> IN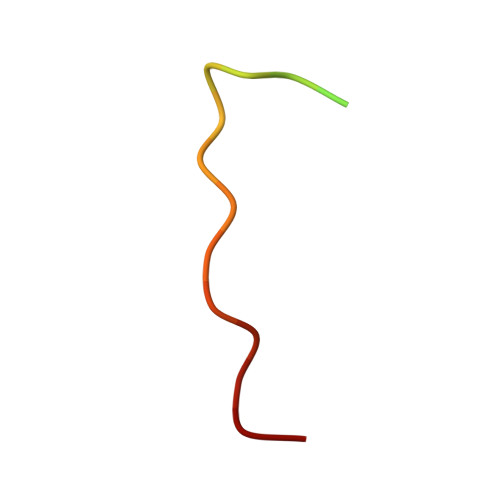TTNAHSTSNILIPELKAPKS>MTETLPPVTESAVALQAEVTQRELFEFVLNDPLLASSLYINIALAGLSILLFVFMTRGLDDPRAKLIAVSTILVPVVSIASYTGLASGLTISVLEMPAGHFAEGSSVMLGGEEVDGVVTMWGRYLTWALSTPMILLALGLLAGSNATKLFTAITFDIAMCVTGLAAALTTSSHLMRWFWYAISCACFIVVLYILLVEWAQDAKAAGTADIFSTLKLLTVVMWLGYPIVWALGVEGVAVLPVGYTSWAYSALDIVAKYI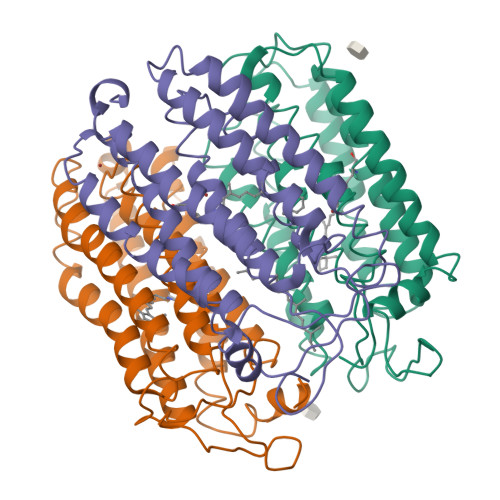FAFLLLNYLTSNEGVVSGSILDVPSASGAPADD[6x]>MSHLRIPKNWTIQRSTPFFTKDNVPEALLTHHNTAVDVFGQICVMEGVVTYYGFANSEATEPEIKVVINAGQFATSPPQYWHRIELSD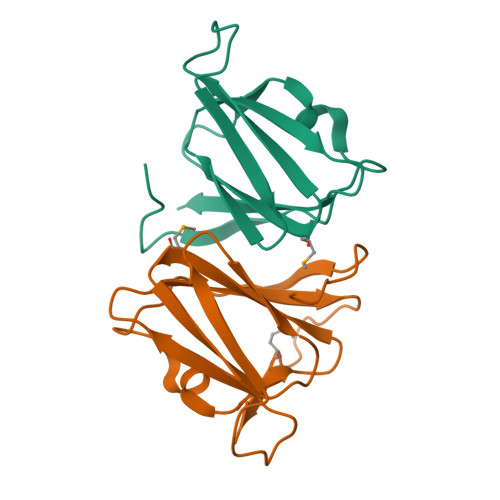DAQFNINFWSDQDKSGKKMFNTKLEHHHHHH[8x]>MQLTPTFYDN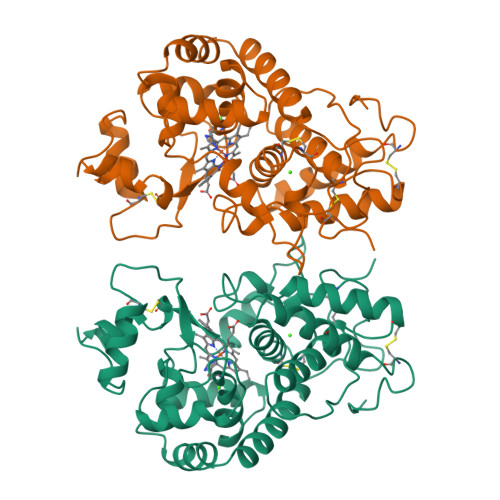SCPNVSNIVRDTIVNELRSDPRIAASILRLHFHDCFVNGCDASILLDNTTSFRTEKDAFGNANSARGFPVIDRMKAAVESACPRTVSCADLLTIAAQQSVTLAGGPSWRVPLGRRDSLQAFLDLANANLPAPFFTLPQLKDSFRNVGLNRSSDLVALSGGHTFGKNQCRFIMDRLYNFSNTGLPDPTLNTTYLQTLRGLCPLNGNLSALVDMDLRTPTIFDNKYYVNLEEQKGLIQSDQELFSSPNATDTIPLVRSFANSTQTFFNAFVEAMDRMGNITPLTGTQGQIRLNCRVVNSNS[2x]>[2x]MLIAFEGIDGSGKTTQAKKLYEYLKQKGYFVSLYREPGGTKVGEVLREILLTEELDERTELLLFEASRSKLIEEKIIPDLKRDKVVILDRFVLSTIAYQGYGKGLDVEFIKNL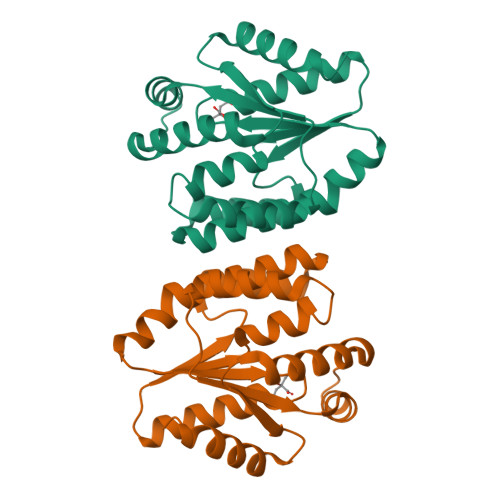NEFATRGVKPDITLLLDIPVDIALRRLKEKNRFENKEFLEKVRKGFLELAKEEENVVVIDASGEEEEVFKEILRALSGVLRV>MTRYQNLVNGKWKSSEQEITIYSPINQEELGTVPAMTQTEADEAMQAARAALPAWRALSAIERAAYLHKTAAILERDKEKIGTILAKEVAKGIKAAIGEVVRTADLIRYAAEEGLRITGQAMEGGGFEAASKNKLAVVRREPVGIVLAIAPFNYPVNLSASKIAPALIAGNVVMLKPPTQGSISGLLLAKAFEEAGIPAGVFNTITGRGSEIGDYIIEHKEVNFINFTGSTPIGERIGRLAGMRPIMLELGGKDAALVLEDADLEHAAKQIVAGAFSYSGQRCTAIKRVIVLESVADKLATLLQEEVSK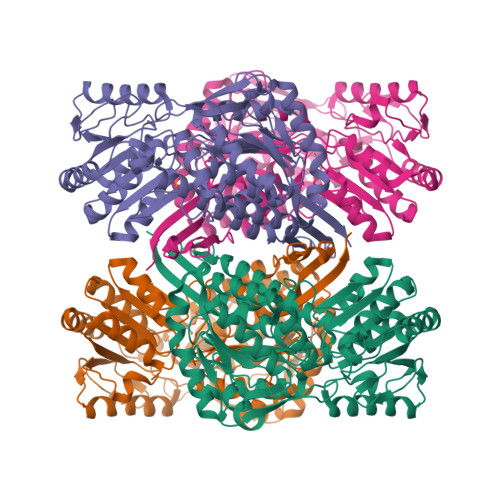LTVGDPFDNADITPVIDNASADFIWGLIEDAQEKEAQALTPIKREGNLLWPVLFDQVTKDMKVAWEEPFGPVLPIIRVASVEEAIAFANESEFGLQSSVFTNDFKKAFEIAEKLEVGTVHINNKTQRGPDNFPFLGVKGSGAGVQGIKYSIEAMTNVKSIVFDVK[4x]> GAE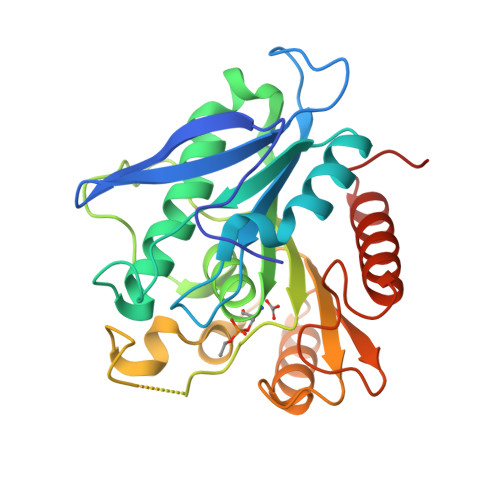VGRLRYPPEMPGAEVKVYKKVDNVDLKLYIYKPADWKPADRRSAIVFFFGGGWQSGSPAQFRPQCEYFAGRGMVAMAADYRVGSRHNVKVADCVADAKSAIRWVRQHAAELGVDPQKIVASGGXAGGHLAACTVMVPDLEAPEEDHTISSQANAAILFNPVLILSREGLKDHVPRQDWEERLRERLGTEPKAVSPYHHIRAGLPPMIIFHGTADNTVPFETIRLFAEAMKKAGNRCELVPFEGAAHGFFNFGRGDNLAYQKTLELADEFLVEIGFLAPKGESQP> DVYQEPTDPKFPQQWYLSGVTQRDLNVKEAWAQGFTGHGIVVSILDDGI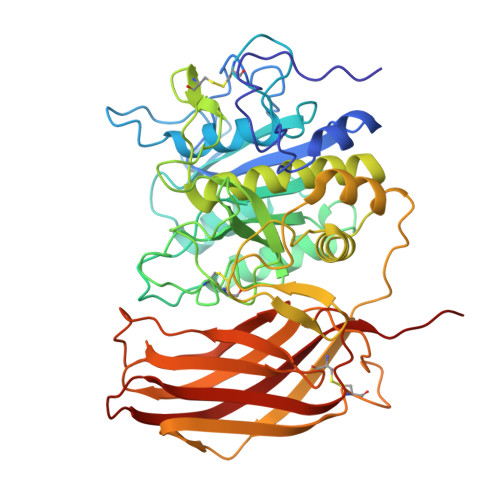EKNHPDLAGNYDPGASFDVNDQDPDPQPRYTQMNDNRHGTRCAGEVAAVANNGVCGVGVAYNARIGGVRMLDGEVTDAVEARSLGLNPNHIHIYSASWGPEDDGKTVDGPARLAEEAFFRGVSQGRGGLGSIFVWASGNGGREHDSCNCDGYTNSIYTLSISSATQFGNVPWYSEACSSTLATTYSSGNQNEKQIVTTDLRQKCTESHTGTSASAPLAAGIIALTLEANKNLTWRDMQHLVVQTSKPAHLNADDWATNGVGRKVSHSYGYGLLDAGAMVALAQNWTTVAPQRKCIVEILVEPKDIGKRLEVRKAVTACLGEPNHITRLEHVQARLTLSYNRRGDLAIHLISPMGTRSTLLAARPHDYSADGFNDWAFMTTHSWDEDPAGEWVLEIENTSEANNYGTLTKFTLVLYGTAPEGL> SMNPFDATAGYRSLTYEEVLQELVKHKELLRRKDTHIRELEDY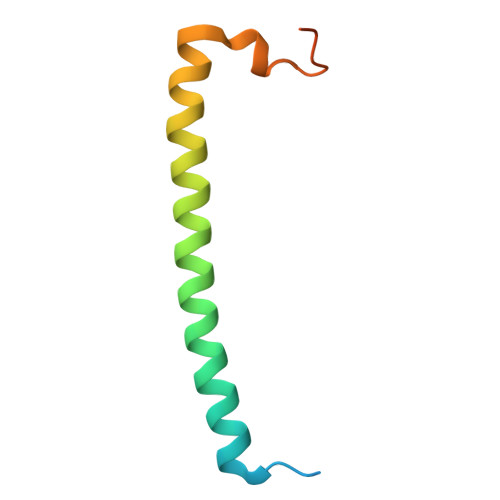IDNLLVRVMEETPSILRVPYEPSRKAGKFSNS>[4x]MASVVGTP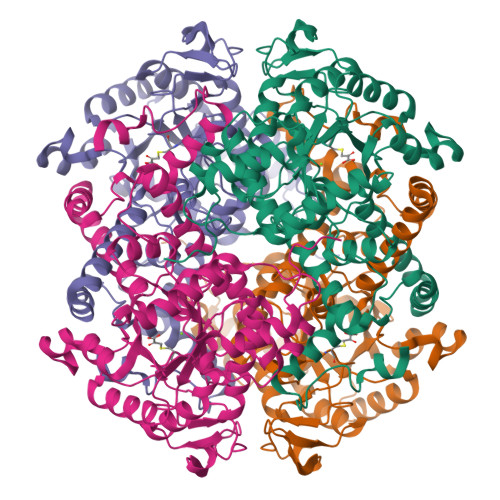KSAEQIQQEWDTNPRWKDVTRTYSAEDVVALQGSVVEEHTLARRGAEVLWEQLHDLEWVNALGALTGNMAVQQVRAGLKAIYLSGWQVAGDANLSGHTYPDQSLYPANSVPQVVRRINNALQRADQIAKIEGDTSVENWLAPIVADGEAGFGGALNVYELQKALIAAGVAGSHWEDQLASEKKCGHLGGKVLIPTQQHIRTLTSARLAADVADVPTVVIARTDAEAATLITSDVDERDQPFITGERTREGFYRTKNGIEPCIARAKAYAPFADLIWMETGTPDLEAARQFSEAVKAEYPDQMLAYNCSPSFNWKKHLDDATIAKFQKELAAMGFKFQFITLAGFHALNYSMFDLAYGYAQNQMSAYVELQEREFAAEERGYTATKHQREVGAGYFDRIATTVDPNSSTTALTGSTEEGQFH> ETHRRVRLLKHGSDKPLGFYIRDGTSVRVTASGLEKQPGIFISRLVPGGLAESTGLLAVNDEVIEVNGIEVAGKTLDQVTDMMVANSSNL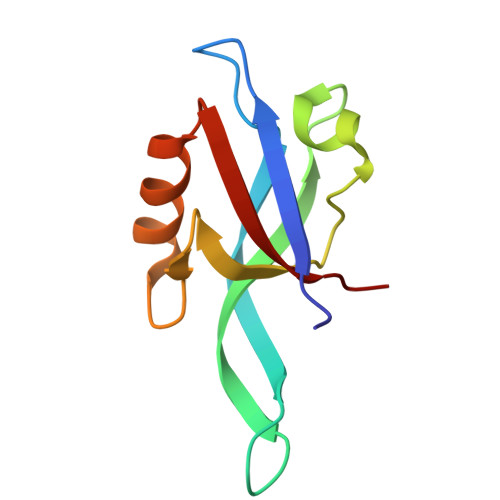IITVKPAN> HHHHHHMMTSKDHVKSQIPRLSAINDLHKIWPTVEEHGAAIIESFLSLDIVRR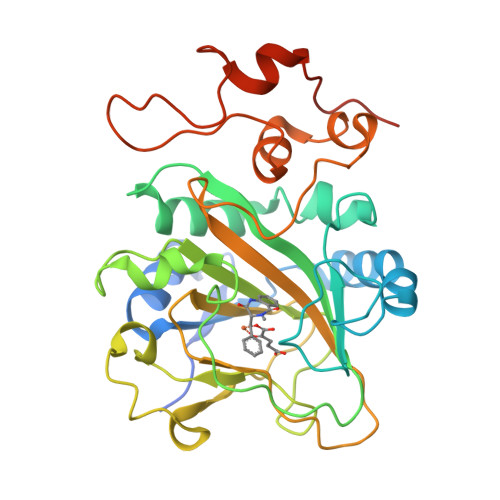LNEEVDPFVKIEPIPAAKTKDHPNHVLSTTTRLVNVLAPISKAYREDVLNSKVLHRICSDAFHVYGDYWVLMGAVMELAPSNPAQPLHRDMRFSHPIVEYLKPDAPATSINFLVALSPFTAENGATHVILGSHKWQNLSNVSMDATVRALMNPGDALLITDSTIHCGGAETTGTETRRLLTITMGISQLTPLESNLAVPRPVIESLTPLAQRLLGWASQRSAAPRDIGLLTIRGNSIEKTMNLKAEQPLHDDEAEPLCRETI> MSETPLLDELEKGPWPSFVKEIKKTAELMEKAAAEGKDVKMPKGARGLLKQLEISYKDKKTHWKHGGIVSVVGYGGGVIGRYSDLGEQIPEVEHFHTMRINQPSGWFYSTKALRGLCDVWEKWGSGLTNFHGSTGDIIFLGTRSEYLQPCFEDLGNLEIPFDIGGSGSDLRTPSACMGPALCEFACYDTLELCYDLTMTYQDELHRPMWPYKFKIKCAGCPNDCVASKARSDFAIIGTWKDDIKVDQEAVKEYASWMDIENEVVKLCPTGAIKWDGKELTIDNRECVRCMHCINKMPKALKPGDERGATILIGGKAPFVEGAVIGWVAVPFVEVEKPYDEIKEILEAIWDWWDEEGKFRERIGELIWRKGMREFLKVIGREADVRMVKAPRNNP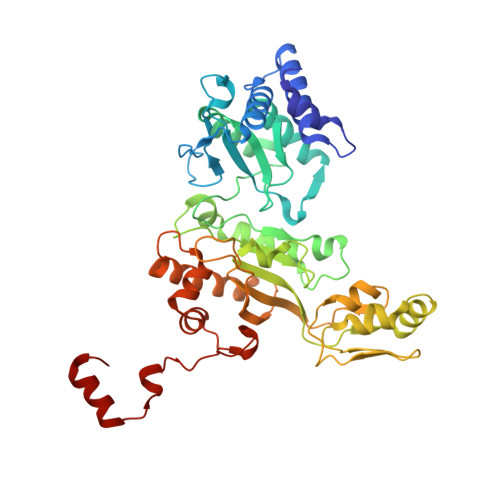FMFFEKDELKPSAYTEELKKRGMW>[4x]GQSAVEAIKQKGKLVVATSPDYAPFEFQSLVDGKNQVVGADIDMAQAIADELGVKLEILSMSFDNVLTSLQTGKADLAVAGISATDERK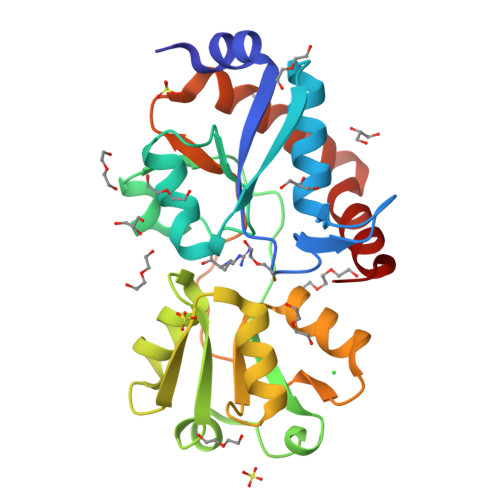EVFDFSIPYYENKISFLVHKADVEKYKDLTSLESANIAAQKGTVPESMVKEQLPKAQLTSLTNMGEAVNELQAGKIDAVHMDEPVALSYAAKNAGLAVATVSLKMKDGDANAVALRKNSDDLKEVVDKVIQKLKDEGTYQSYLEKAASLTEVEE> SDSSRRQYQEKYKQVEQYMSFHKLPPDTRQRIHDYYEHRYQGKMFDEESILGELSEPLREEIINFNCRKLVASMPLFANADPNFVTSMLTKLRFEVFQPGDYIIREGTIGKKMYFIQHGVVSVLTKGNKETK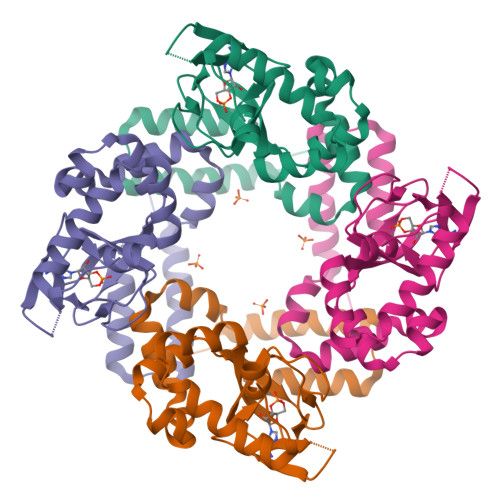LADGSYFGEICLLTRGRRTARVRADTYCRLYSLSVDNFNEVLEEYPMMRRAFETVALDRLDRIGKKNSILLHK>SMVPYVPTPKPVVDRMLELADVDETDVLYDLGSGDGRIVIRAARTHGARGVGIEIDPDLVKKARKNAKEAGVADLVEFRQGDLFEADISEA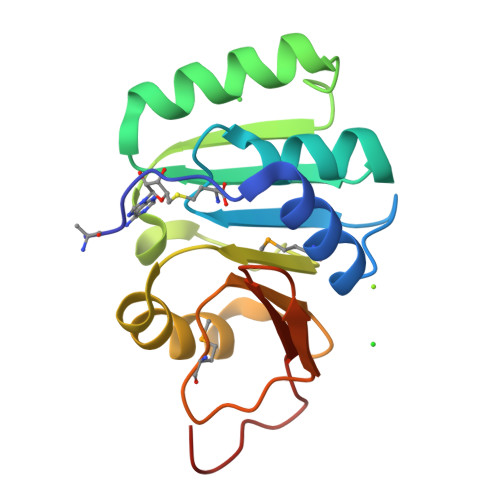TVVTLYLLPSVNQKLRPILFEQLSPGTPVVSHDFDMGRWAPDRTVDLEGDTVYRWTIPEEIPEDLDE[2x]> MTRIISIVSGKGGTGKTTVTANLSVALGEMGRKVLAVDGDLTMANLSLVLGVDDVNITLHDVLAGDAKLEDAIYMTQFENVYILPGAVDWEHVIKADPRKLPEVIKSLKGKYDFILIDCPAGLQLRAMSAMLSGEEAILVTNPEISCLTDTMKVGMVLKKAGLAILGFILNRYGRSERDIPPEAAQDVMDVPLLAVIPEDPVIREGT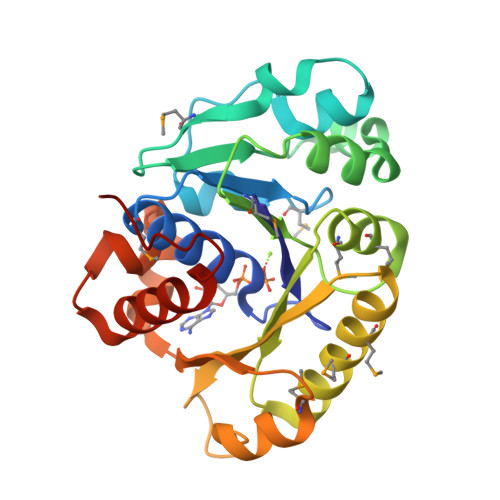LEGIPAVKYKPESKGAQAFIKLAEEVDKLAGIKAKI>MMQQSRPASDPQVVEAARKEGRLIIYSSTDQSSAQALLDDFRKLYPFIQIEYNDLGTQAIYDRFVSETAAGASSADLLWSSAMELQVKLASEGYALPYDSPEAKNWPANARLGNLAYSTTLEPAVVVYNKRFLKPEEVPTTREGLARLLQEPRMRGRVATWDPERSAVGFTILKADYDRFPAFQELARAFGKAQAALYSSTGAAFEKVISGEHYLAYGFFGSYALLRQRTVKDLGIAYLTDGTVAIQRVAFINKRAAHPNAAKLFLDYLLSLRGQNLMAYTALIFARRETVVGE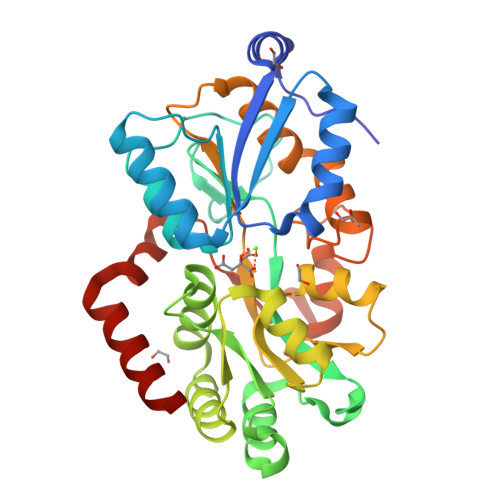ATPQALYKAVGGKDKVYAIPVSTEILKNLDPAERMRFLTFWRQAVRGQ[2x]~{N}-ethyl-4-[5-[1-(2-hydroxyethyl)pyrazol-4-yl]benzimidazol-1-yl]-2,6-dimethoxy-benzamide | C23 H25 N5 O4 | 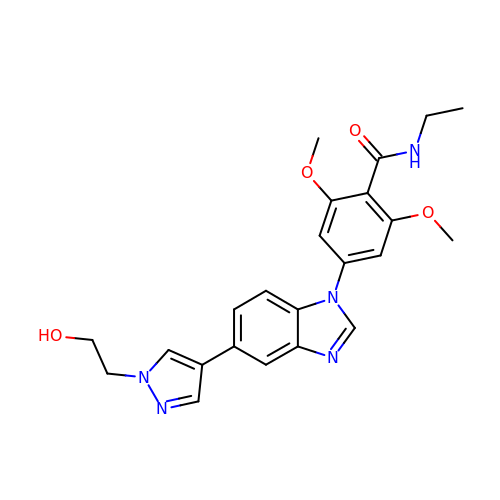FCJGMZMSVIAAJU-UHFFFAOYSA-N>SQANLMRLKSDLFNRSPMYPGPTKDDPLTVTLGFTLQDIVKVDSSTNEVDLVYYEQQRWKLNSLMWDPNEYGNITDFRTSAADIWTPDITAYSSTRPVQVLSPQIAVVTHDGSVMFIPAQRLSFMCDPTGVD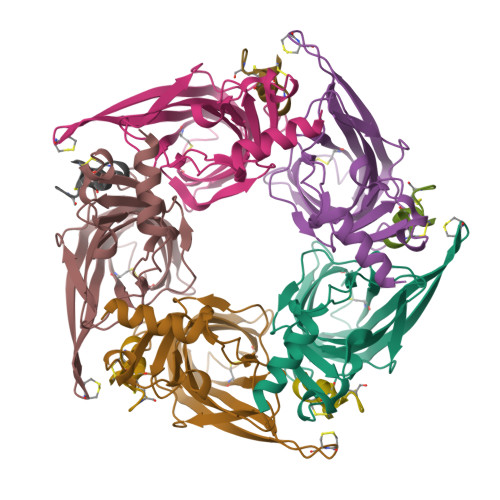SEEGVTCAVKFGSWVYSGFEIDLKTDTDQVDLSSYYASSKYEILSATQTRQVQHYSCCPEPYIDVNLVVKFRERR[5x];>GCCSHPACAVDHPEICX[5x]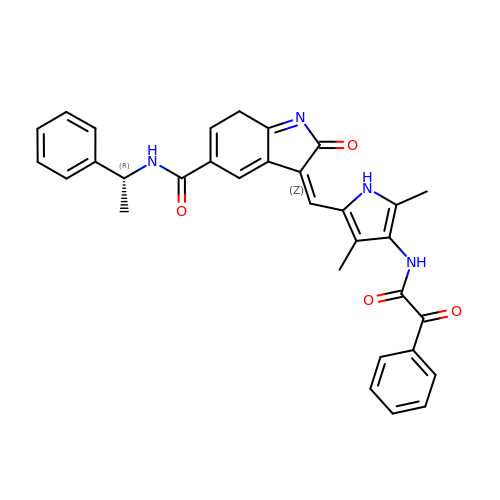(3Z)-3-{[3,5-dimethyl-4-(2-oxo-2-phenylacetamido)-1H-pyrrol-2-yl]methylidene}-2-oxo-N-[(1R)-1-phenylethyl]-3,7-dihydro-2H-indole-5-carboxamide | C32 H28 N4 O4 | LYBBCQSHMUMOJF-DWGAWOTKSA-N> ACGCAGCCTGTACGGACATCA;> CCGT;> TCTGATGT;> GGCTGC;> ACA;> G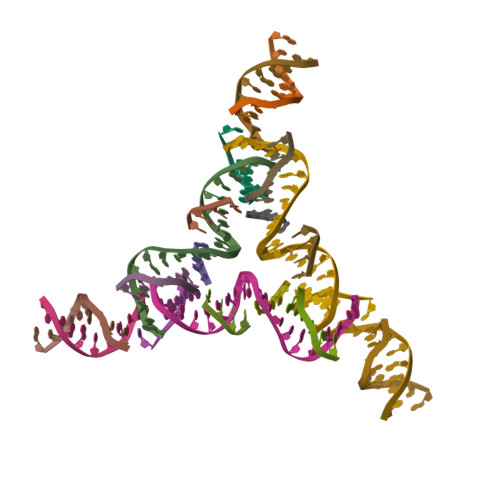TACTCAGCA;> GATGCTGAGT> HHHHHHGSMTIPDVFPHLPLIAITRNPVFPRFIKIIEVKNKKLVELLRRKVRLAQPYVGVFLKRDDSNESDVVESLDEIYHTGTFAQIHEMQDLGDKLRMIVMGHRRVHISRQLEVEPEEPEAENKHKPRRKSKRGKKEAEDELSARHPAELAMEPTPELPAEVLMVEVENVVHEDFQVTEEVKALTAEIVKTIRDIIALNPLYRESVLQMMQAGQRVVDNPIYLSDMGAALTGAESHELQDVLEETNIPKRLYKALSLLKKEFELSKLQQRLGREVEEKIKQTHRKYLLQEQLKIIKKELGLEKDDKDAIEEKFRERLKELVVPKHVMDVVDEELSKLGLLDNHSSEFNVTRNYLDWLTSIPWGKYSNENLDLARAQAVLEEDHYGMEDVKKRILEFIAVSQLRGSTQGKILCFYGPPGVGKTSIARSIARALNREYFRFSVGGMTDVAEIKGHRRTYVGAMPGKIIQCLKKT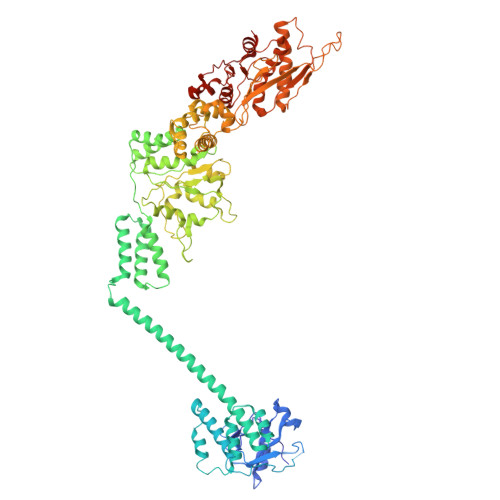KTENPLILIDEVDKIGRGYQGDPSSALLELLDPEQNANFLDHYLDVPVDLSKVLFICTANVTDTIPEPLRDRMEMINVSGYVAQEKLAIAERYLVPQARALCGLDESKAKLSSDVLTLLIKQYCRESGVRNLQKQVEKVLRKSAYKIVSGEAESVEVTPENLQDFVGKPVFTVERMYDVTPPGVVMGLAWTAMGGSTLFVETSLRRPQDKDAKGDKDGSLEVTGQLGEVMKESARIAYTFARAFLMQHAPANDYLVTSHIHLHVPEGATPKDGPSAGCTIVTALLSLAMGRPVRQNLAMTGEVSLTGKILPVGGIKEKTIAAKRAGVTCIVLPAENKKDFYDLAAFITEGLEVHFVEHYREIFDIAFPDEQAEALAVER>AESHWCYEVQAESSNYPCLVPVKWGGNCQKDRQSPINIVTTKAKVDKKLGRFFFSGYDKKQTWTVQNNGHSVMMLLENKASISGGGLPAPYQAKQLHLHWSDLPYKGSEHSLDGEHFAMEMHIVHEKEKGTSRNVKEAQDPEDEIAVLAFLVEAGTQVNEGFQPLVEALSNIPKPEMSTTMAESSLLDLLPKEEKLRHYFRYLGSLTTPTCDEKVVWTVFREPIQLHREQILAFSQKLYYDKEQTVSMKDNVRPLQQLGQRTVIK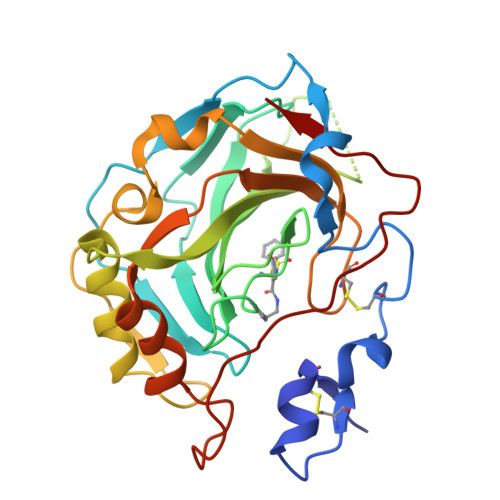S[2x]>KQMVLADIRSIGTNTIDVYPGNDFGDDDPQYQQALKYDDLIAIQKQPWVASATPAVSQNLRLRYNNVDVAASANGVSGDYFNVYGMTFSEGNTFNQEQLNGRAQVVVLDSNTRRQLFPHKADVVGEVILVGNMPARVIGVAEEKQSMFGS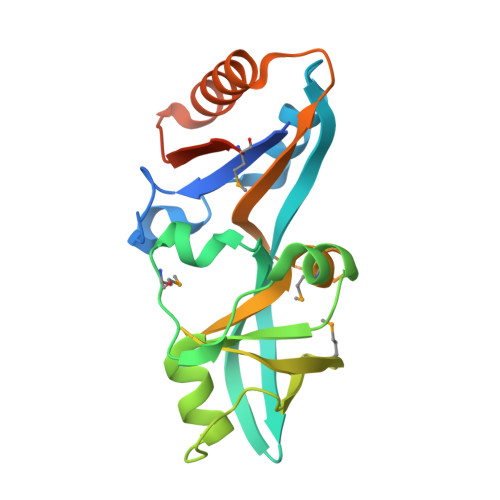SKVLRVWLPYSTMSGRVMGQSWLNSITVRVKEGFDSAEAEQQLTRLLSLRHGKKDFFTWNMDGVLKTVEKTTRTLQ[7x]> LAMPAAERLMQEKGVSPAEVQGTG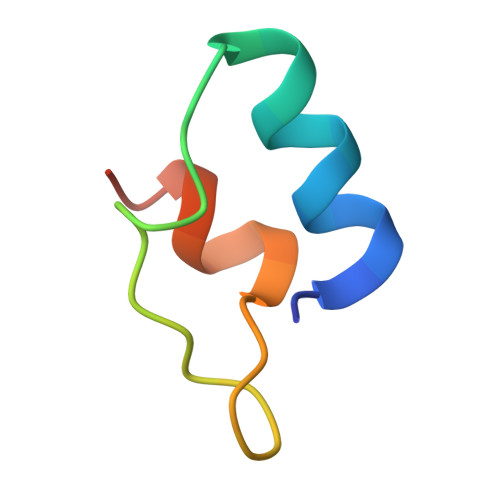LGGRILKEDVMRHLEE> EEPPKEKLHTLEEFSYEFFRAPEKDMVSMAVLPLARARGHLWAYSCEPLRQPLLKRVHANVDLWDIACQIFVAILRYMGDYPSRQAWPTLELTDQIFTLALQHPALQDEVYCQILKQLTHNSNRHSEERGWQLLWLCTGLFPPSKGLLPHAQKFIDTRRGKLLAPDCSRRIQKVLRTGPRK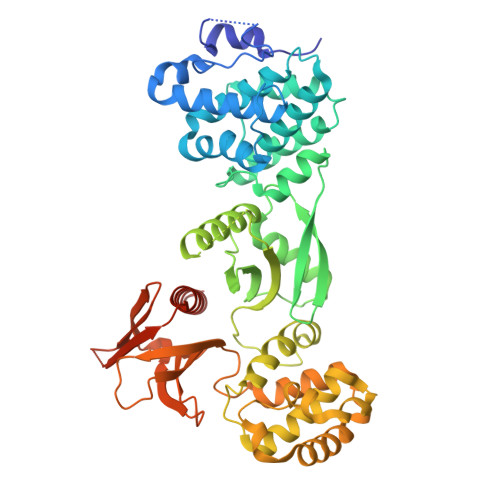QPPHQVEVEAAEQNVSRICHKIYFPNDTSEMLEVVANTRVRDVCDSIATRLQLASWEGCSLFIKISDKVISQKEGDFFFDSLREVSDWVKKNKPQKEGAPVTLPYQVYFMRKLWLNISPGKDVNADTILHYHQELPKYLRGFHKCSREDAIHLAGLIYKAQFNNDRSQLASVPKILRELVPENLTRLMSSEEWKKSILLAYDKHKDKTVEEAKVAFLKWICRWPTFGSAFFEVKQTSEPSYPDVILIAINRHGVLLIHPKTKDLLTTYPFTKISSWSSGSTYFHMALGSLGRGSRLLCETSLGYKMDDLLTSYVQQLLSAMNKQRGSKAPALAST>GPGSMVPRVPQPGIWCPAVTFFDSKTDTLDLASQERYYAYLARSGLTGLVILGTNAEAFLLTREERAQLIATARKAVGPDFPIMAGVGAHSTRQVLEHINDASVAGANYVLVLPPAYFGKATTPPVIKSFFDDVSCQSPLPVVIYNFPGVCNGIDLDSDMITTIARKNPNVVGVKLTCASVGKITRLAATLPPAAFSVFGGQSDFLIGGLSVGSAGCIAAFANVFPKTVSKIYELYKAGKVDQAMELHRKAALAESPCKSGIATTKYAAAIFSAKAAGIEDAE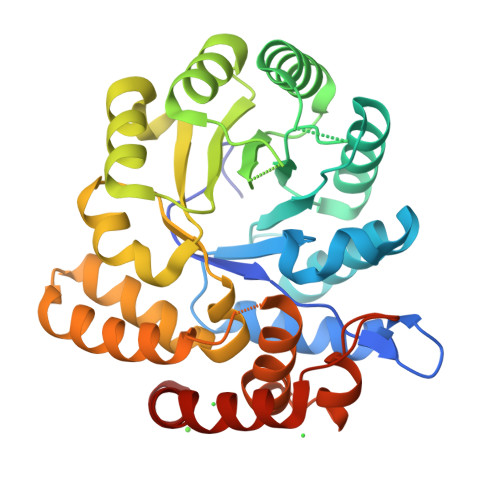EKLRPRKPYDPPSEAAKQEVRKVMAEVAAIEAGLS[2x]(2R)-3-HYDROXY-2-METHYLPROPANOIC 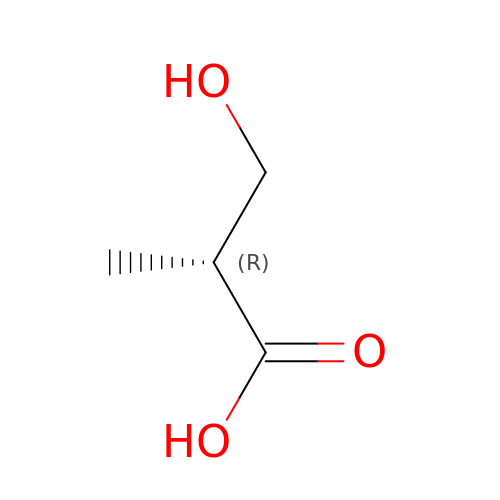ACID | C4 H8 O3 | DBXBTMSZEOQQDU-GSVOUGTGSA-N>GHMAEAFYEELKEKADIGEVAGDAIVSFQDVFFTTPRGRY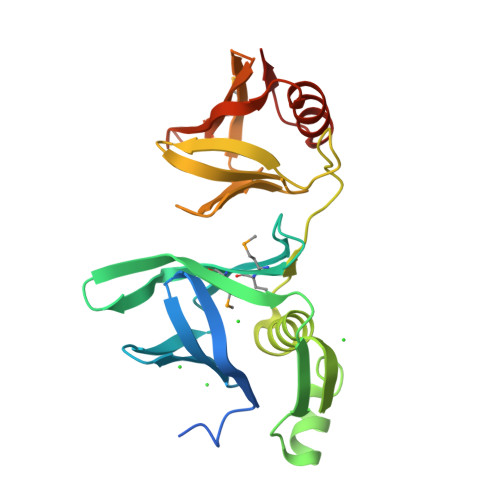DIDIYKNSIRLRGKTYEYKLQHRQIQRIVSLPKADDIHHMMVMAIEPPLRQGQTTYPFLVLQFQKDEETEVQLNLEDEDYEENYKDKLKKQYDAKTHIVLSHVLKGLTDRRVIVPGEYKSKYDQCAVSCSFKANEGYLYPLDNAFFFLTKPTLYIPFSDVSMVNISRAGQTSTSSRTFDLEVVLRSNRGSTTFANISKEEQQLLEQFLKSKNLRVKNEDRE[2x]>[2x]TDPIADMLTRIRNATRVYKESTDVPASRFKEEILRILAREGFIKGYERVDVDGKPYLRVYLKYGPRRQGPDPRPEQVIHHI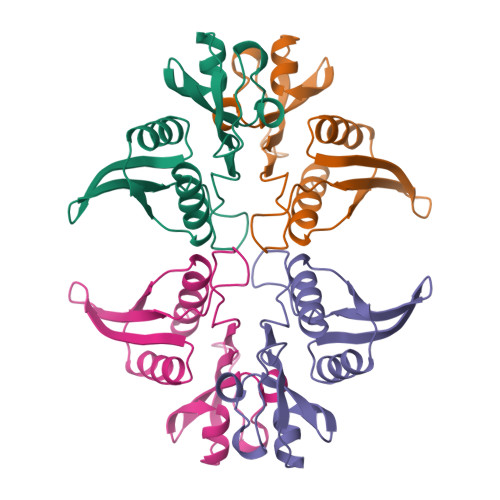RRISKPGRRVYVGVKEIPRVRRGLGIAILSTSKGVLTDREARKLGVGGELICEVW> MGSPASDPTVFHKRYLKKIRDLGEGHFGKVSLYCYDPTNDGTGEMVAVKALKADAGPQHRSGWKQEIDILRTLYHEHIIKYKGCCEDAGAASLQLVMEYVPLGSLRDYLPRHSIGLAQLLLFAQQICEGMAYLHAQHYIHRDLAAR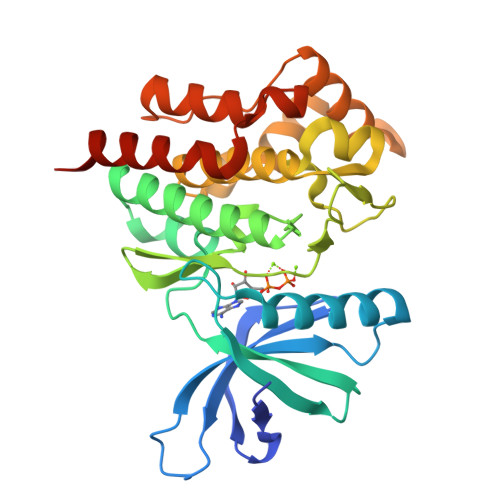NVLLDNDRLVKIGDFGLAKAVPEGHEYYRVREDGDSPVFWYAPECLKEYKFYYASDVWSFGVTLYELLTHCDSSQSPPTKFLELIGIAQGQMTVLRLTELLERGERLPRPDKCPAEVYHLMKNCWETEASFRPTFENLIPILKTVHEKYRHHHHHH3-(benzyloxy)aniline | C13 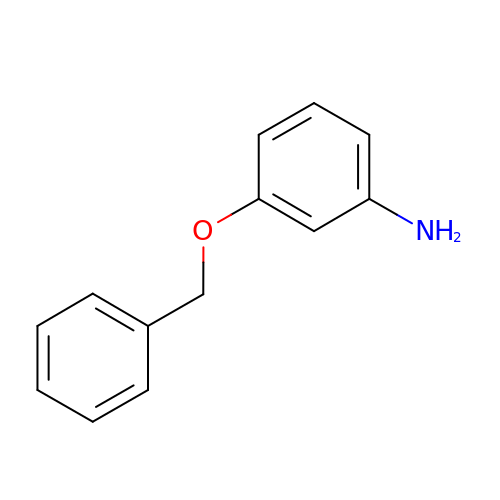H13 N O | IGPFOKFDBICQMC-UHFFFAOYSA-N3-{(1R)-1-[(3-methyl-4-{[6-(trifluoromethyl)pyridin-3-yl]methyl}-1H-pyrrole-2-carbonyl)amino]ethyl}-1H-pyrazole-5-carboxamide | C19 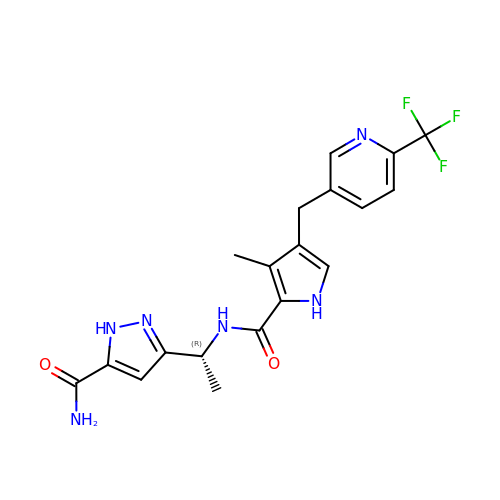H19 F3 N6 O2 | YOVYZOJIMZERTC-SNVBAGLBSA-N> GSEVAIKMVVVGNGAVGKSSMIQRYCKGIFTKDYKKTIGVDFLERQIQVNDEDVRLMLWDTAGQEEFDAITKAYYRGAQACVLVFST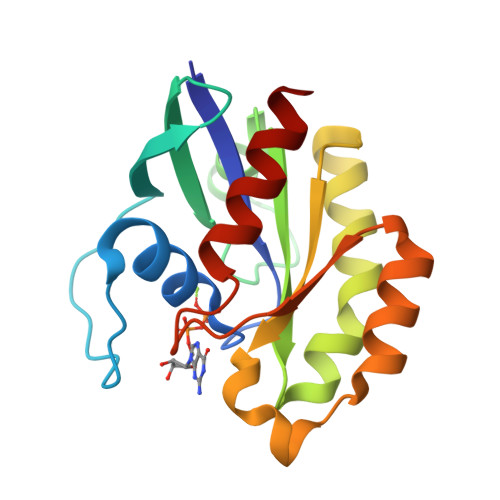TDRESFEAISSWREKVVAEVGDIPTALVQNKIDLLDDSCIKNEEAEGLAKRLKLRFYRTSVKEDLNVSEVFKYLAEKHLQK>SNIMSTSGTGKMTRAQRRAAARRNRRTAGVQPVIVEPIAAGQGKAIKAIAGYSISKWEASSDAITAKATNAMSITLPHELSSEKNKELKVGRV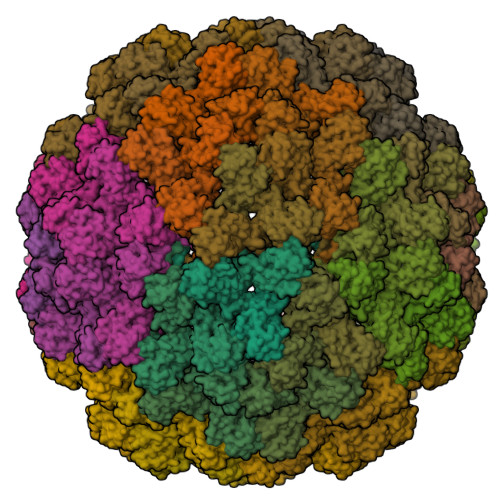LLWLGLLPSVAGRIKACVAEKQAQAEAAFQVALAVADSSKEVVAAMYTDAFRGATLGDLLNLQIYLYASEAVPAKAVVVHLEVEHVRPTFDDFFTPVYK[180x]6-(2-ethyl-4-hydroxyphenyl)-N-(6-methylpyridin-3-yl)-1H-indazole-3-carboxamide 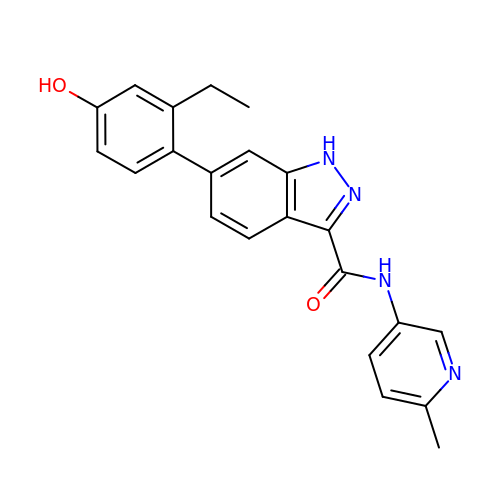| C22 H20 N4 O2 | CUKXYSDQFPFABZ-UHFFFAOYSA-N> DMLPEIAAAVGFLSSLLRTRGCVSEQRLKVFSGALQEALTEHYKHHWFPEKPSKGSGYRCIRINHKMDPIISRVASQIGLSQPQLHQLLPSELTLWVDPYEVSYRIGEDGSICVLYEE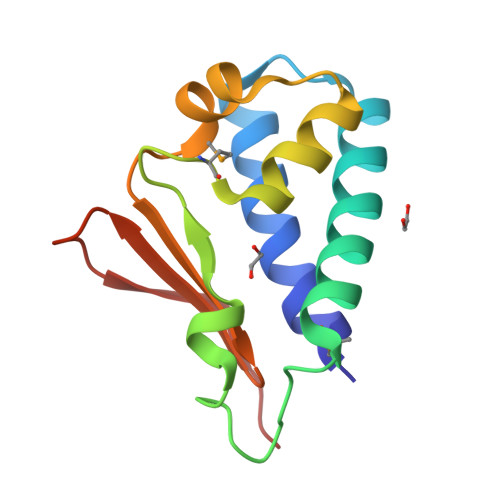AP>SNAMKFELPKLPYAVDALESTISKETIEYHYGKHHQTYVTNLNNLVEGTEHDGRNLEEIVKTSNGGIFNNA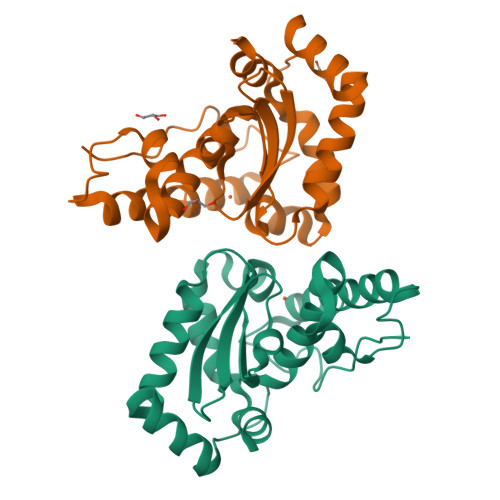AQVFNHTFYWNCLTPNKTEASSQLKAALIETFGSVENFKEQFSKAAIATFGSGWAWLVKNTEGKLEIVTTSNAGCPLTENKKPLLTFDVWEHAYYIDYRNARPKYVEALWDIVNWQFVSEQFAD[2x]>MEKIKYLKSIQISQRSVLDLELLAVGAFTPLDRFMGEEDYRNVVESMRLKSGTLFPIPITLPMEKEIAKDLKEGEWIVLRDPKNVPLAIMRVEEVYKWNLEYEAKNVLGTTDPRHPLVAEMHTWGEYYISGELKVIQLPKYYDFPEYRKTPKQVREEIKSLGLDKIVAFQTRNPMHRVHEELTKRAMEKVG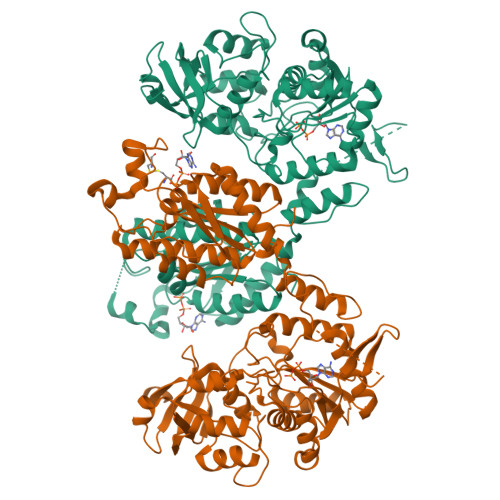GGLLLHPVVGLTKPGDVDVYTRMRIYKVLYEKYYDKKKTILAFLPLAMRMAGPREALWHGIIRRNYGATHFIVGRDHASPGKDSKGKPFYDPYEAQELFKKYEDEIGIKMVPFEELVYVPELDQYVEINEAKKRNLKYINISGTEIRENFLKQGRKLPEWFTRPEVAEILAETYVPKHKQGFCVWLTGLPCAGKSTIAEILATMLQARGRKVTLLDGDVVRTHLSRGLGFSKEDRITNILRVGFVASEIVKHNGVVICALVSPYRSARNQVRNMMEEGKFIEVFVDAPVEVCEERDVKGLYKKAKEGLIKGFTGVDDPYEPPVAPEVRVDTTKLTPEESALKILEFLKKEGFIKD[2x]>[2x]PNFSGNWKIIRSENFEELLKVLGVNVMLRKIAVAAASKPAVEI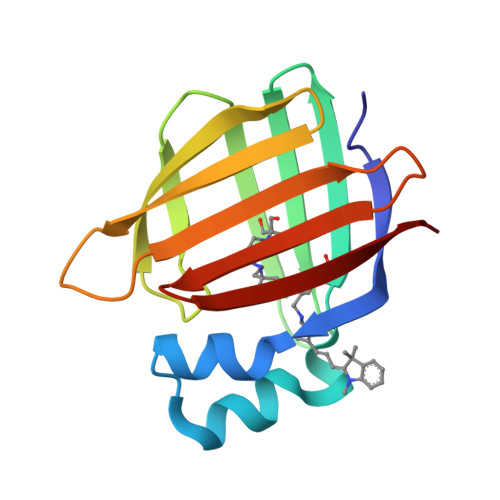KQEGDTFYIKTSTTVRTTEINFKVGEEFEEQTVDGRPCKSLVKWESENKMVCEQKLLKGEGPKTSWTLELTNDGELIDTMTADDVVCTKVYVRE>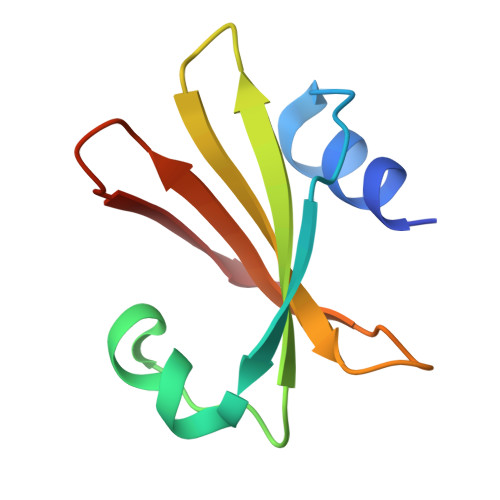 MTNLSDIIEKETGKQLVIQESILMLPEEVEEVIGNKPESDILVHTAYDESTDENVMLLTSDAPEYKPWALVIQDSNGENKIKML> XAAP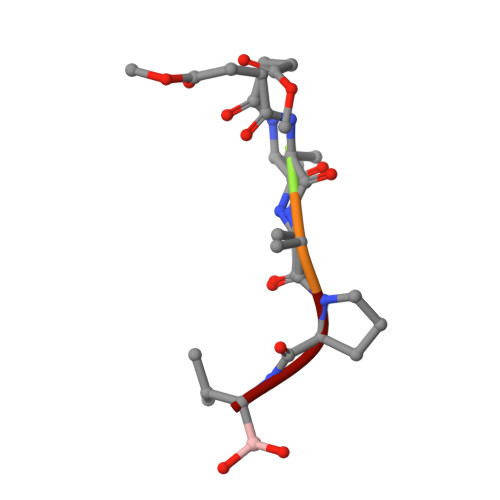V> AYTTFSQTKNDQLKEPMFFGQPVNVARYDQQKYDIFEKLIEKQLSFFWRPEEVDVSRDRIDYQALPEHEKHIFISNLKYQTLLDSIQGRSPNVALLPLISIPELETWVETWAFSETIHSRSYTHIIRNIVNDPSVVFDDIVTNEQIQKRAEGISSYYDEL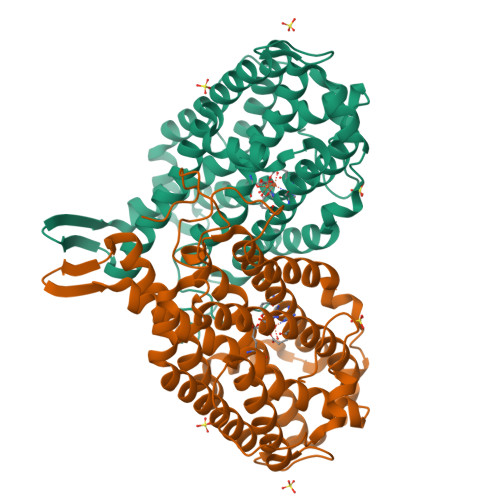IEMTSYWHLLGEGTHTVNGKTVTVSLRELKKKLYLCLMSVNALEAIRFYVSFACSFAFAERELMEGNAKIIRLIARDEALHLTGTQHMLNLLRSGADDPEMAEIAEECKQECYDLFVQAAQQEKDWADYLFRDGSMIGLNKDILCQYVEYITNIRMQAVGLDLPFQTRSNPIPWINTWLVSDNVQVAPQEVEVSSYLVGQIDSEVDTDDLSNFQL> MASMTGGQQMG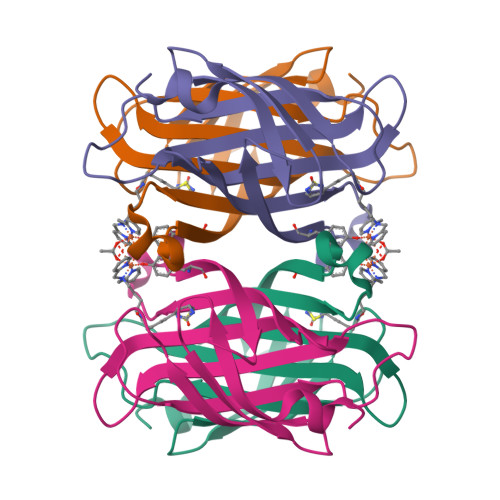RDEAGITGTWYNQLGSTFIVTAGADGALTGTYESAVGNAESRYVLTGRYDSAPATDGSGTALGWTVAWKNNYRNAHSATTWSGQYVGGAEARINTQWLLTSGTTEANAWASTYVGHDTFTKVKPSAASIDAAKKAGVNNGNPLDAVQQ>DYKDDDDKAEVKKIPTMIEGFDDISHGGLPQGATTLVSGTSGTGKTLFAVQFLYNGITIFNEPGIFVTFEESPQDIIKNALSFGWNLQSLIDQGKLFILDASPDPDGQEVAGDFDLSALIERIQYAIRKYKATRVSIDSVTAVFQQYDAASVVRREIFRLAFRLAQLGVTTIMTTERVDEYGPVARFGVEEFVSDNVVILRNVLEGERRRRTVEILKLRGTTHMKGEYPFTINNGINIFDYKDDDDK[2x];>[2x]MAPLRKTAVLKLYVAGNTPNSVRALKTLNNILEKEFKGVYALKVIDVLKNPQLAEEDKILATPTLAKVLPPPVRRIIGDLSNREKVLIALRLLAEEIGD;>DYKDDDDKSNVDPQHRLSQKLKERLGYLGVYYKRDTAFFFRRMSPADKRKLLDELRSIYRTIVLEYFNTDAKVNERIDEFVSKAFFADISVSQVLEIHVELMDTFSKQLKL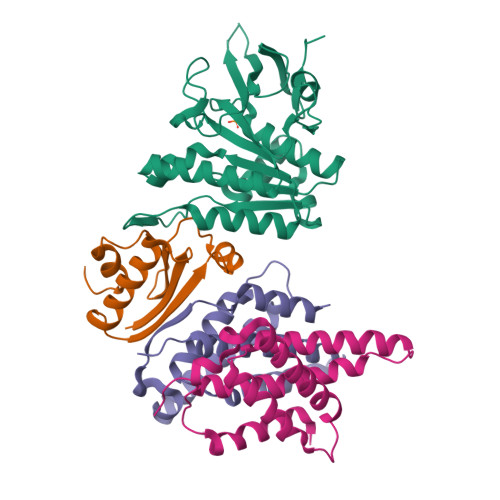EGRSEDILLDYRLTLIDVIAHLSEMYRRSIPREV[4x]>[3x]M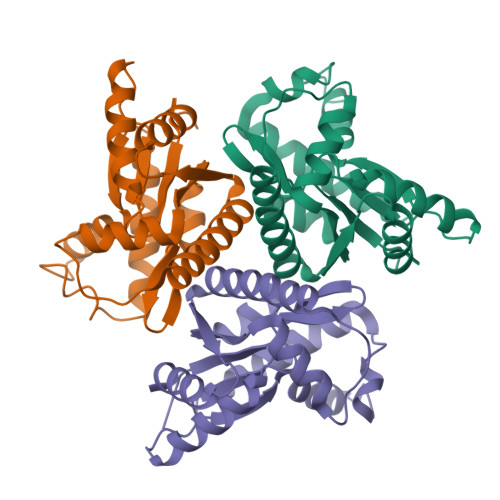KNKLVVVTGVPGVGGTTITQKAMEKLSEEGINYKMVNFGTVMFEVAQEENLVEDRDQMRKLDPDTQKRIQKLAGRKIAEMVKESPVVVDTHSTIKTPKGYLPGLPVWVLNELNPDIIIVVETSGDEILIRRLNDETRNRDLETTAGIEEHQIMNRAAAMTYGVLTGATVKIIQNKNNLLDYAVEELISVLR Glyceraldehyde-3-phosphate dehydrogenase (GAPDH) is a highly conserved enzyme involved in the ubiquitous process of glycolysis and presents a loop (residues 208–215 of Escherichia coli GAPDH) in two alternative conformations (I and II). In the presence of inorganic phosphate (Pi), GAPDH catalyzes the conversion of D-glyceraldehyde-3-phosphate (G3P) to 1,3-diphosphoglycerate (BPG), accompanying the reduction of NAD+ to NADH. All the structures reported in this paper have four subunits: O, P, Q, and R. Each subunit contained two domains: the C-terminal catalytic domain and the N-terminal NAD+-binding domain. Two anion recognition sites, “Ps” and “Pi”, bind the C3 phosphate of G3P and inorganic phosphate, respectively.

The structure of ternary complexes H177A.NAD.BPG and C150S.NAD.NPG provides further information on the driving force behind the phosphorylation step and the mechanism of the nucleophilic attack of inorganic phosphate on the carbonyl group of the thioacyl intermediate to generate BPG. In addition, the O subunit of C150S.NAD.BPG and the P subunit of H177A.NAD.BPG contain an unexpectedly large electron-dense cluster near the active site and NAD+, which was attributed to the product BPG. BPG in C150S.NAD.BPG and H177A.NAD.BPG holds refined occupancy factors of 0.85 and 0.8, respectively. Upon the superimposition of the ternary complexes C150S.NAD.BPG and H177A.NAD.BPG with their corresponding binary complexes, the RMSD values are 0.104 (1197 atoms) and 0.168 Å (1235 atoms), respectively. These results indicate that the overall structures of H177A.NAD.BPG and C150S.NAD.BPG are like those of its binary complex, except for the presence of the product. BPG is observed in a released state in H177A.NAD.BPG. The oxygen atom of O5P of C3 phosphate forms hydrogen bonds with NH1 of Arg232 and with Oγ of Thr182 and Thr180. O6P and O7P form hydrogens with 2′-OH of NAD+ ribose and Oγ of Thr182 and water, respectively. The oxygen atom O3P of the C1 phosphate is stabilized by three hydrogen bonds interacting with the amide nitrogen of Gly210 and with H2O 551 and H2O 689.

>[4x]HHHHHHSSGLVPRGSHMASMSKVGINGFGRIGRLVLRRLLEVKSNIDVVAINDLTSPKILAYLLKHDSNYGPFPWSVDFTEDSLIVDGKSIAVYAEKEAKNIPWKAKGAEIIVECTGFYTSAEKSQAHLDAGAKKVLISAPAGEMKTIVYNVNDDTLDGNDTIVSVASCTTNCLAPMAKALHDSFGIEVGTMTTIAAYTGTQSLVDGPRGKDLRASRAAAENIIPHTTGAAKAIGLVIPELSGKLKGHAQRVPVKTGSVTELVSILGKKVTAEEVNNALKQATTNNESFGYTDEEIVSSDIIGSHFGSVFDATQTEITAVGDLQLVKTVAWYDNEYGFVTQLIRTLEKFAKL1-[(3~{R})-3-(4-azanyl-3-ethynyl-pyrazolo[3,4-d]pyrimidin-1-yl)piperidin-1-yl]prop-2-en-1-one | 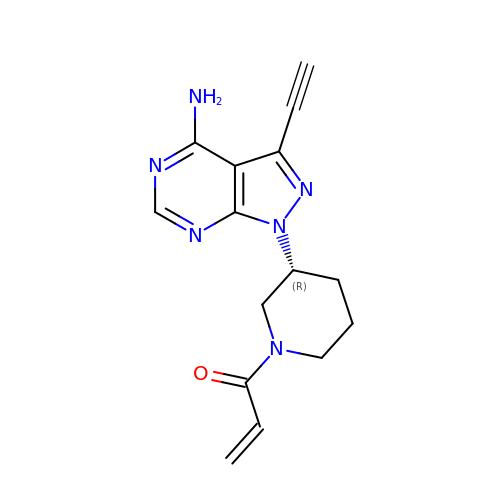C15 H16 N6 O | XXFDMGXYEIKFNZ-SNVBAGLBSA-N methyl 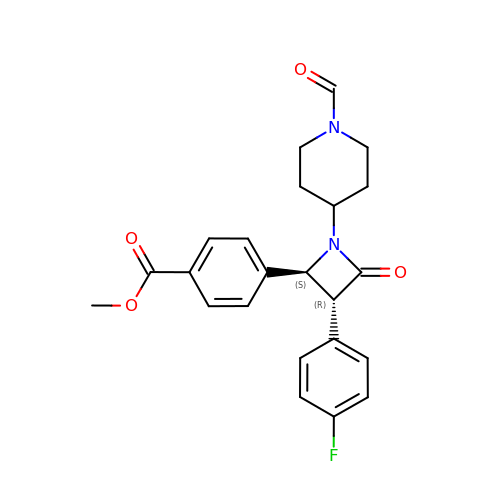4-[(2~{S},3~{R})-3-(4-fluorophenyl)-1-(1-methanoylpiperidin-4-yl)-4-oxidanylidene-azetidin-2-yl]benzoate | C23 H23 F N2 O4 | WIVVLBDUDQXNLC-RTWAWAEBSA-N>MSDKDSKNTPQVPEKLGLSRRGFLGASAVTGAAVAATALGGAVMTRESWAQAVKESKQKIHVGPGELDDYYGFWSGGHQGEVRVLGVPSMRELMRIPVFNVDSATGWGLTNESRHIMGDSAKFLNGDCHHPHISMTDGKYDGKYLFINDKANSRVARIRLDIMKCDKMITVPNVQAIHGLRLQKVPHTKYVFANAEFIIPHPNDGKVFDLQDENSYTMYNAIDAETMEMAFQVIVDGNLDNTDADYTGRFAAATCYNSEKAFDLGGMMRNERDWVVVFDIHAVEAAVKAGDFITLGDSKTPVLDGRKKDGKDSKFTRYVPVPKNPHGCNTSSDGKYFIAAGKLSPTCSMIAIDKLPDLFAGKLADPRDVIVGEPELGLGPLHTTFDGRGNAYTTLFIDSQVVKWNMEEAVRAYKGEKVNYIKQKLDVHYQPGHLHASLCETNEADGKWLVALSKFSKDRFLPVGPLHPENDQLIDISGDEMKLVHDGPTFAEPHDCIMARRDQIKTKKIWDRNDPFFAPTVEMAKKDGINLDTDNKVIRDGNKVRVYMT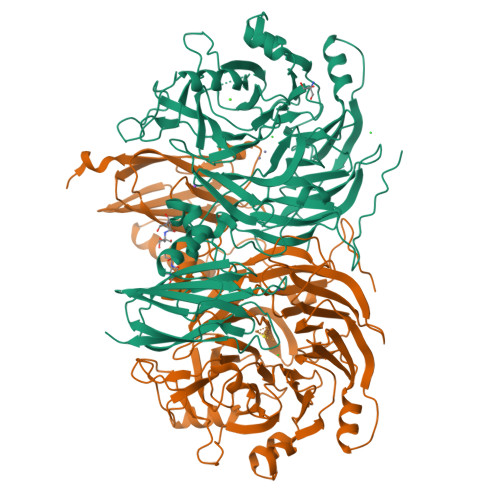SMAPAFGVQEFTVKQGDEVTVTITNIDQIEDVSNGFVVVNHGVSMEISPQQTSSITFVADKPGLHWYYCSWFCHALHMEMVGRMMVEPAWSHPQFEK[2x]>MTVAKAIFIKCGNLGTSMMMDMLLDERADREDVEFRVVGTSVKMDPECVEAAVEMALDIAEDFEPDFIVYGGPNPAAPGPSKAREMLADSEYPAVIIGDAPGLKVKDEMEEQGLGYILVKPDAMLGARREFLDPVEMAIYNADLMKV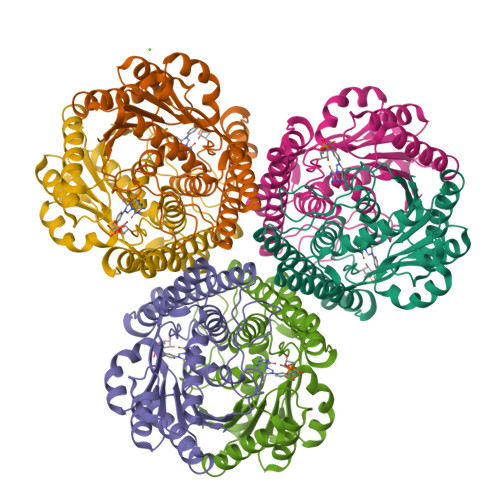LAATGVFRVVQEAFDELIEKAKEDEISENDLPKLVIDRNTLLEREEFENPYAMVKAMAALEIAENVADVSVEGCFVEQDKERYVPIVASAHEMMRKAAELADEARELEKSNDAVLRTPHAPDGKVLSKRKFMEDPE[12x]> GDVQNAVEGAMVRVADTVQTSATNSERVPNLTAVETGHTSQAVPGDTMQTRHVINNHVRSESTIENFLARSACVFYLEYKTGTKEDSNSFNNWVITTRRVAQLRRKLEMFTYLRFDMEITVVITSSQDQSTSQNQNAPVLTHQIMYVPPGGPIPVSVDDYSWQTSTNPSIFWTEGNAPARMSIPFISIGNAYSNFYDGWSHFSQAGVYGFTTLNNMGQLFFRHVNKPNPAAITSVARIYFKPKHVRAWVPRPPRLCPYINSTNVNFEPKPVTEVRTNIITT;> GYSDRVRSITLGNSTITTQECANVVVGYGEWPEYLSDNEATAEDQPTQPDVATCRFYTLDSVQWENGSPGWWWKFPDALRDMGLFGQNMYYHYLGRAGYTIHVQCNASKFHQGCILVVCVPEAEMGSAQTSGVVNYEHISKGEIASRFTTTTTAEDHGVQAAVWNAGMGVGVGNLTIFPHQWINLRTNNSATIVMPYVNSVPMDNMYRHHNFTLMIIPFVPLDFSAGASTYVPITVTVAPMCAEYNGLRLAGHQ;> GLPT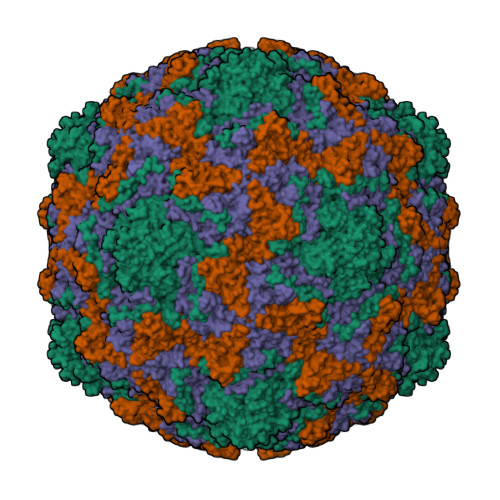MNTPGSNQFLTSDDFQSPSAMPQFDVTPEMHIPGEVRNLMEIAEVDSVMPINNDSAAKVSSMEAYRVELSTNTNAGTQVFGFQLNPGAESVMNRTLMGEILNYYAHWSGSIKITFVFCGSAMTTGKFLLSYAPPGAGAPKTRKDAMLGTHVVWDVGLQSSCVLCIPWISQTHYRFVEKDPYTNAGFVTCWYQTSVVSPASNQPKCYMMCMVSACNDFSVRMLRDTKFIEQTSFYQ;> GAQVSTQKTGAHETSLSATGNSIIHYTNINYYKDAASNSANRQDFTQDPGKFTEPMKDVMIKTLPALN> GGSDIRPDIKDDIYDPTYADAAGPSPKVEYVWRNIILMSLLHLGALYGITLIPTCKFYTWLWGVFYYFVSALGITAGAHRLWSHRSYKARLPLRLFLIIANTMAFQNDVYEWARDHRAHHKFSETHADPHNSRRGFFFSHVGWLLVRKHPAVKEKGSTLDLSDLEAEKLVMFQRRYYKPGLLMMCFILPTLVPWYFWGETFQNSVFVATFLRYAVVLNATWLVNSAAHLFGYRPYDKNISPRENILV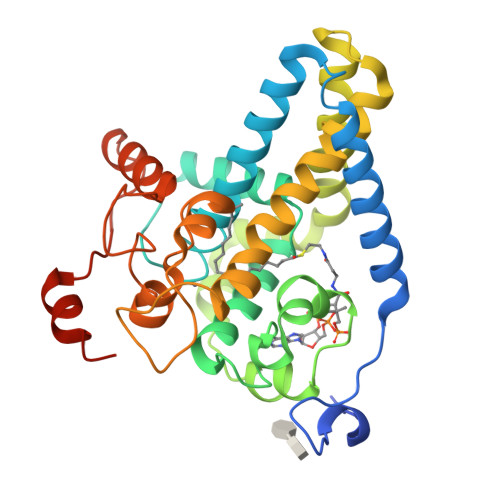SLGAVGEGFHNYHHSFPYDYSASEYRWHINFTTFFIDCMAALGLAYDRKKVSKAAILARIKRTGDGNYKSG>MDYYYSLISPPCQSAILLAKKLGITLNLKKTNVHDPVERDALTKLNPQHTIPTLVDNGHVVWESYAIVLYLVETYAKDDTLYPKDPKVRSVVNQRLFFDIGTLYKRIIDVIHLVMKKEQPSDEQMEKLKGALDLLEQFVTERAYAAADHLTVADICLLGTV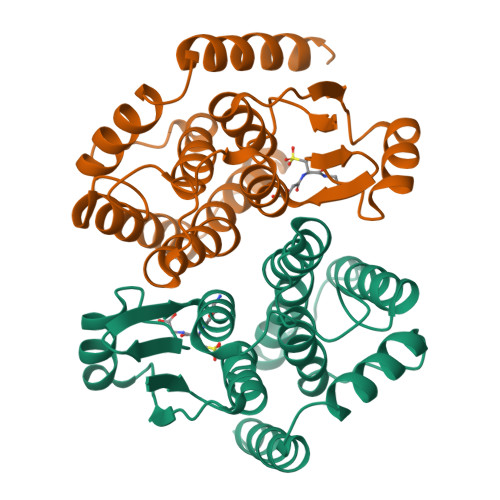TALNWLKHDLEPFPHIRAWLERVRAEMPDYEEFSKQVADDTLAYVASRK[4x]> SNAMSKDSESNLAQRQSQPKAHADLRINSHWIIPIENTTDHNLVSNILIDHCLLIKDGIILAIEPQSSCQIPATETLDLGQQVLMPGWVNAHGHAAMSLFRGLADDLPLMTWLQEHVWPAEAQHVDEHFVKQGTELAIAEMIQSGTTTFADMYFYPQQSGEAALAAGIRAVCFAPVLDFPTNYAQNADEYIRKAIECNDRFNNHPMNEQGLVQIGFGPHAPYTVSDEPLKEITMLSDQLDMPVQIHLHETDFEVSESLETFNKRPTQ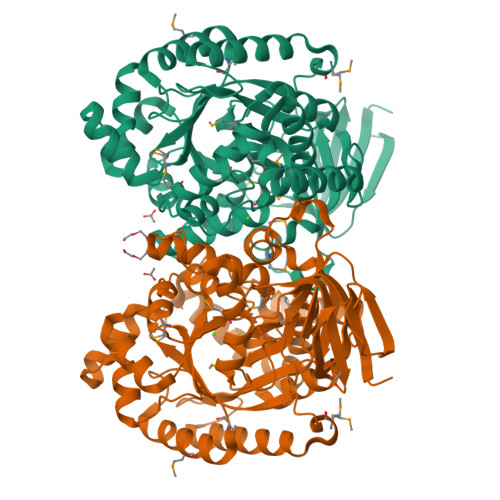RLADIGFLNERVSCVHMTQVDDGDIKILQKTGASIIHCPESNLKLASGFCPIAKLSAANIPLAIGTDGAASNNDLDMFSETKTAALLAKGVSQDASAIPAIEALTMATLGGARALGIDDITGSLKPGKAADIQAIDLNTLSSQPVFDPVSHMVYCTKSTQVSHVWVNGRCLLKNGELTTLNEETLINHAKAWASAIRTPIK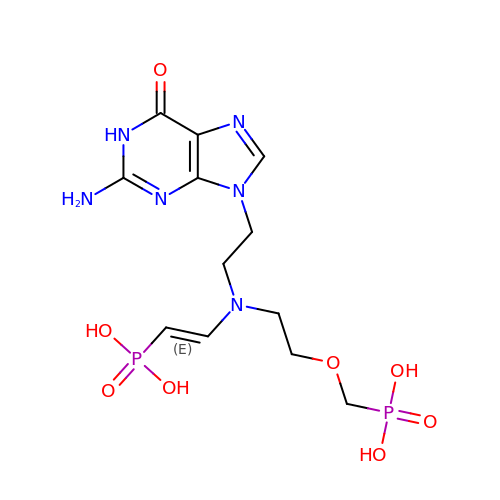[(2-{[2-(2-amino-6-oxo-1,6-dihydro-9H-purin-9-yl)ethyl][(E)-2-phosphonoethenyl]amino}ethoxy)methyl]phosphonic acid | C12 H20 N6 O8 P2 | HGNAMUIMUCHWJL-GQCTYLIASA-N>MKEWQENKSWNAHFTEHKSQGVVVLWNENKQQGFTNNLKRANQAFLPASTFKIPNSLIALDLGVVKDEHQVFKWDGQTRDIATWNRDHNLITAMKYSVVPVYQEFARQIGEARMSKMLHAFDYGNEDISGNVDSFWLDGGIRISATEQISFLRKLYHNKLHVSERSQRIVKQAMLTEANGDYIIRAKTGYSPKIGWWVGWVELDDNVWFFAMNMDMPTSDGLGLRQAITKEVLKQEKIIPLEHHHHHHHH[2x]

One of the main carbapenemases is the class D β-lactamase OXA-48, which represents a major public health threat because of its rapid spread worldwide. Although OXA-48 hydrolyzes penicillins at high level, it hydrolyzes carbapenems at a low level and shows very weak activity against expanded-spectrum cephalosporins. OXA-405 is a peculiar OXA-48-like enzyme, as it has lost carbapenem activities and gained expanded-spectrum cephalosporin hydrolytic activity subsequent to a 4 amino-acid (AA) deletion in the β5–β6 loop. Kinetic parameters confirmed that OXA-405 behaves more like an ESBL ß-lactamase, rather than a carbapenemase.

The crystal structure of OXA-405 refined at 2.26 Å presents the typical class D fold with an α-helical region and a mixed α-helix/β-sheet region, with 96% of all residues inside the favored regions of the Ramachandran plot, 4% in the allowed regions, and no outliers. The asymmetric unit contains two protein chains, A and B, modeled with 246 residues each. The crystal structure of OXA-405 showed that the 213-TRIE-217 deletion did not modify the overall structure of the protein but resulted in an important decrease of the size of the β5–β6 loop, with important consequences on the overall shape of the binding site. Clear electron density is observed for both backbones and side chains, including the active site and the β5–β6 loop, with the exception of side chains of Lys218 (OXA-48 numbering) from the β5–β6 loop and of Met22 (not shown). The Lys218 is flexible, as shown by the reduced electron density observed on this side chain. In contrast, the R2 substituent of cephalosporins has unfavorable steric clashes with Arg214 in OXA-48 that are not observed in OXA-405, where this residue is absent and the β5–β6 loop is shorter. These structural differences explain the systematically lower Km values of cephalosporins in the complex with OXA-405 compared with those of OXA-48. OXA-405 features a more open conformation of the active site due to the absence of Arg214 and its stabilizing interaction with Asp159, as well as the smaller size of the β5–β6 loop. This leads to an increased affinity for cephalosporins and a decreased stabilization of carbapenems in the active site, thus explaining the important differences in affinity for these substrates observed between OXA-48 and OXA-405. Our results confirm, that the four AA deletion in the β5–β6 loop observed in OXA-405 is responsible for a drastic loss of carbapenemase activity, particularly for imipenem, and a gain of cephalosporinase activity with the ability to hydrolyze cefotaxime and ceftazidime.> MDGEGFGELLQQAEQLAAETEGVTELPHVERNLQEIQQAGERLRSKTMTRTSQESANVKASVLLGSRGLDISHISQRLESLSAATTFEPLEPVKDTDIQGFLKNEKDNALLSAIEESRKRTFVMAEEYHRESMLVEWEQVKQRVLHTLLASGEDALDFTQESETSYISESGAPGRSSLDNVEMAYARQMYMYNEKVVSGHLQPSLVDLCTEAAERLDDKNVSDLWVMVKQMTDVPLIPASDTLKSRCSGQMQMAFVRQALNYLEQSYKNYTLISVFANLQQAQLGGVPGTYNLVRSFLNIRLPTPIPGLQDGEIEGYPVWALIYYCMRCGDLMAAQQVVNRAQHQLGDFKNCFQE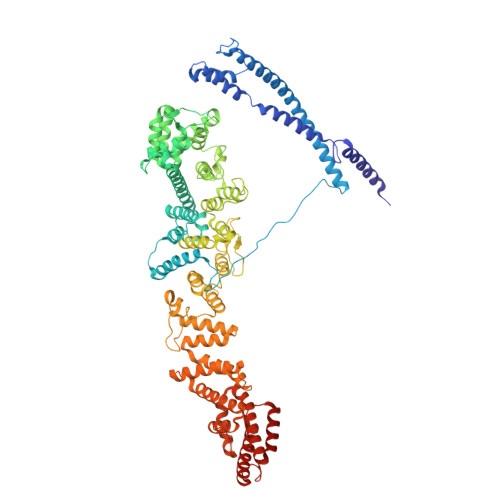YIHNKDRRLSPTTENKLRLHYRRAVRASTDPYKRAVYCIIGRCDVSDNHSEVADKTEDYLWLKLSQVCFEDEANSSPQDRLTLPQFQKQLFEDYGESHFAVNQQPYLYFQVLFLTAQFEAAIAFLFRLERTRCHAVHVALALFELKLLLKSTGQSAQLLSQEPGEPQGVRRLNFIRLLMLYTRKFEPTDPREALQYFYFLRNEKDNQGESMFLRCVSELVIESREFDMLLGKLEKDGSRKPGAIDKFTRDTKTIINKVASVAENKGLFEEAAKLYDLAKNPDKVLELTNKLLSPVVSQISAPQSNRERLKNMALAIAERYKSQGVSAEKSINSTFYLLLDLITFFDEYHAGHIDLSFDVIERLKLVPLSQDSVEERVAAFRNFSDEIRHNLSEILLATMNILFTQYKRLKGSGPTTLGRPQRVQEDKDSVLRSQARALITFAGMIPYRMSGDTNARLVQMEVLMN>GSHMASDLLELTEDMEKEISNALGHGPQDEILSSAFKLRITRGDIQTLKNYHWLNDEVINFYMNLLVERNKKQGYPALHVFSTFFYPKLKSGGYQAVKRWTKGVNLFEQEIILVPIHRKVHWSLVVIDLRKKCLKYLDSMGQKGHRICEILLQYLQDESKTKRNSDLNLLEW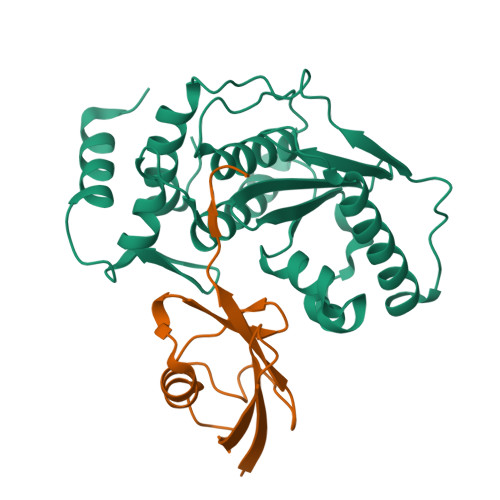THHSMKPHEIPQQLNGSDSGMFTCKYADYISRDKPITFTQHQMPLFRKKMVWEILHQQLL[3x];>GSHMNDHINLKVAGQDGSVVQFKIKRHTPLSKLMKAYCERQGLSMRQIRFRFDGQPINETDTPAQLEMEDEDTIDVFQQQTGGVPESSLAGHSF[3x]> TVPDNLKKQLAVSVRNIQWSYGIFWSVSASQPGVLEWGDGYYNGDIKTRKTIQAAEVKIDQLGLERSEQLRE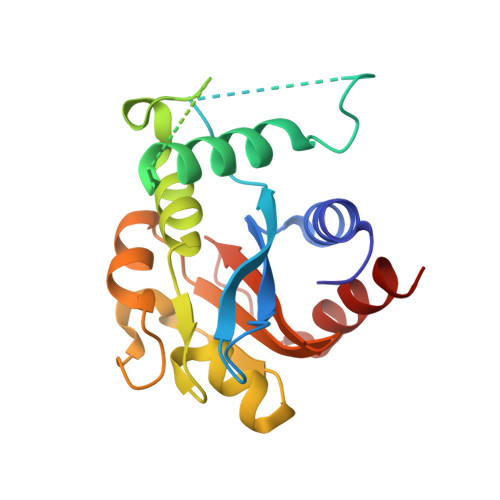LYESLSLAESSASGSSQVTRRASAAALSPEDLTDTEWYYLVCMSFVFNIGEGIPGGALSNGEPIWLCNAETADSKVFTRSLLAKSASLQTVVCFPFLGGVLEIGTTEHIKEDMNVIQSVKTLFLEA> SRKKMGLLVMAFGTPYKEEDIERYYTHIRRGRKPEPEMLQDLKDRYEAIGGISPLAQITEQQAHNLEQHLNEIQDEITFKAYIGLKHIEPFIEDAVAEMHKDGITEA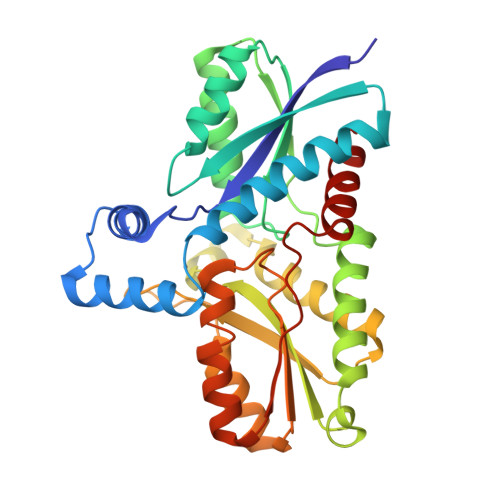VSIVLAPHFSTFSVQSYNKRAKEEAEKLGGLTITSVESWYDEPKFVTYWVDRVKETYASMPEDERENAMLIVSAHSLPEKIKEFGDPYPDQLHESAKLIAEGAGVSEYAVGWQSEGNTPDPWLGPDVQDLTRDLFEQKGYQAFVYVPVGFVADHLEVLYDNDYECKVVTDDIGASYYRPEMPNAKPEFIDALATVVLKKLGR1-(5-fluoro-2-{methyl[3-(methylamino)propyl]amino}pyrimidin-4-yl)-N-[(imidazo[1,2-a]pyridin-3-yl)methyl]azetidine-3-carboxamide | C21 H27 F N8 O | 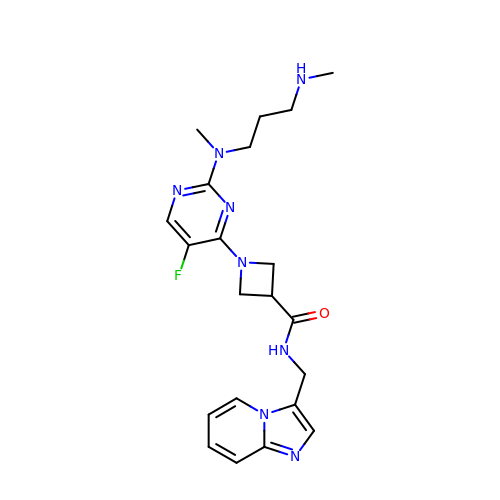BEIRHRPFAQSBMM-UHFFFAOYSA-N> HSNEKWFHGKLGAGRDGRHIAERLLTEYCIETGAPDGSFLVRESETFVGDYTLSFWRNGKVQHCRIHSRQDAGTPKFFLTDNLVFDSLYDLITHYQQVPLRCNEFEMRLSEPVPQTNAHESKEWYHASLTRAQAEHMLMRVPRDGAFLVRKRNEPNSYAISFRAEGKIKHCRVQQEGQTVMLGNSEFDSLVDLISYYEKHPLYRKMKLRYPINEEALEKIGTAEPDYG;>DDLYEEVLFPRN[2x]

Kaposi Sarcoma-associated herpesvirus (KSHV) causes three human malignancies, Kaposi Sarcoma (KS), Primary Effusion Lymphoma (PEL) and the plasma cell variant of multicentric Castleman’s Disease (MCD), as well as an inflammatory cytokine syndrome (KICS). Its non-structural membrane protein, pK15, is among a limited set of viral proteins expressed in KSHV-infected KS tumor cells. Following its phosphorylation by Src family tyrosine kinases, pK15 recruits phospholipase C gamma 1 (PLCγ1) to activate downstream signaling cascades such as the MEK/ERK, NFkB and PI3K pathway, and thereby contributes to the increased proliferation and migration as well as the spindle cell morphology of KSHV-infected endothelial cells. PLCγ1 is a member of the phospholipase C family, which includes several enzymes that hydrolyze phosphatidylinositol 4,5-biphosphate (PIP2) to two important second messengers, inositol 1,4,5-triphosphate (IP3) and diacylglycerol (DAG). Activation of PLCγ1 occurs due to the intramolecular binding of the phosphorylated Y783 to the cSH2 domain, which leads to conformational changes in the protein and the release of the cSH2 domain from the catalytic core of PLCγ1, thus rendering the latter accessible to the substrate PIP2.

We reasoned that the linker region separating the PLCγ1 cSH2 and SH3 domains could have interfered with the binding of the pK15 12mer peptide to the PLCγ1 cSH2 domain, since the former contains tyrosine residue 783, which is known to interact with the PLCγ1 cSH2 domain. We therefore expressed and purified a truncated PLCγ1 tSH2 domain (PLCγ1 aa 545–772), which lacks this linker segment. We obtained diffraction quality crystals of this truncated tSH2 domain in complex with the 12mer phosphorylated pK15 peptide. The structure was determined by the molecular replacement method and refined to a resolution of 2.1Å. In the PLCγ1 cSH2 domain the pK15 peptide straddles the triple ß-sheet that divides the two pockets of the SH2 domain. Its phosphorylated tyrosine residue (pK15 Y481) is in contact with PLCγ1 R675 and R694 in the first of these two pockets, while its hydrophobic residues V484 and L485 in the canonical pK15 SH2-binding site (YEEVL) are in proximity to the second pocket that is known to accommodate hydrophobic residues. The pK15 peptide adopts a similar position to that of residues 781–790 in the PLCγ1 linker peptide containing phosphorylated Y783, which connects the PLCγ1 tSH2 and SH3 domains. The unphosphorylated Y783 sidechain in the cSH2-SH3 linker segment is oriented away from the phosphotyrosine-binding pocket of the cSH2 domain, while the phosphorylated Y783 sidechain superposes well with the K15Y481 side chain. We therefore propose that, following phosphorylation of pK15 on Y481, the last 12 amino acids of the pK15 cytoplasmic domain engage the PLCγ1 cSH2 domain in a manner similar to the PLCγ1 tSH2-SH3 domain linker, once the latter has been phosphorylated on Y783 by the activating receptor tyrosine kinase.>[2x]GSHMVGETQRRFVLKQLDGQTAMPNVPYTITMANGEVIEGVTDAEGATQLLQKDAMNIAKVDMKHTKSPASAVAGIAAAVGAAVAVGKLLGGPDAEAGRALSEGEISLAKGVFGDSIDYSTVRLRDEDYVPWQGKDYVMAPNGHIYFGEELRGVADWSLESLQRQGLFIHEMTHVWQHQHGVNVLLVGAYQQARQFLLGDQYAYRLEPGKTLKDYNIEQQGDIVRDYFLAANAFGEASANSRFAGVLKNFPTGY

Beyond its canonical trimeric spike-forming region containing gp27- and gp5-like domains, VgrG2b harbors a C-terminal extension, rendering it an evolved VgrG protein. The C-terminal portion of the VgrG2b spike protein is predicted to function as a metallopeptidase because of the presence of a signature zinc-binding HEXXH motif. In this work, we find that the VgrG2b C-terminal domain (VgrG2bC-ter) elicits toxicity in the bacterial periplasm, counteracted by a cognate immunity protein. The toxicity of VgrG2bC-ter results in profound morphological anomalies characterized by blebbing of the bacterial membrane at the site of septation, a phenotype reminiscent of inhibition of the cell division machinery by β-lactam antibiotics.

We solved the structure of VgrG2bC-ter, encompassing residues 833–1,019, using crystals of both the native and the selenomethionine-substituted forms with resolutions of 3.2 and 3.0 Å, respectively. Two copies of VgrG2bC-ter were found in the asymmetric unit of the crystal, which could be superimposed with a root-mean-square deviation (RMSD) of 0.1 Å. In solution, however, the purified metallopeptidase domain exists predominantly as a monomer, as determined by size-exclusion chromatography-multi-angle laser light scattering (SEC-MALLS), with a dimeric species also present. The VgrG2bC-ter protomer possesses a single domain composed of six α helices and three β strands, forming a shallow bowl with multiple small loops. A PDB search using the DALI server identified several thermolysin-like metallopeptidases as structural homologs of the VgrG2bC-ter effector domain. One such metallopeptidase is human angiotensin-converting enzyme 2 (Z score: 5.0, Cα RMSD of 4.2 Å across 105 residues), with the active sites of these proteins displaying similar architectures. Although metallopeptidases target diverse substrates, the overall core fold of three α helices (α2, α3, and α5) and two β strands (β2 and β3) is highly conserved and bears the classical HEXXH catalytic motif typical of these zinc-dependent enzymes, where X is any amino acid. Indeed, the conformations of the HEXXH residues in our structure are suggestive of metal ion coordination, and the geometry suggests that the electron density in the putative metal-binding site corresponds to a divalent cation such as zinc. The assigned zinc ion is coordinated by the two histidine residues of the catalytic triad and has a third glutamate ligand (E983) at the top of helix α5. These features permit classification of VgrG2bC-ter as a thermolysin-like gluzincin within the MA(E) metallopeptidase subclan (Rawlings et al., 2018).>MKNITIYTKNYCPYSKKA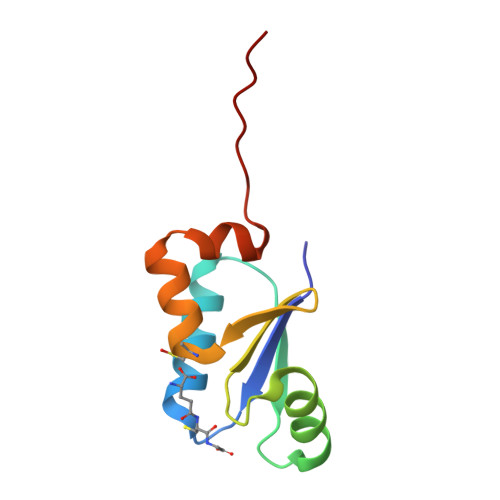VSLLSSKGVDFKEVDVTHDSKAFEDVMAKTGWDTVPQVFVDEEFLGGCDDIHALDRQGILDKKLGLKLEHHHHH[2x]>MGHHHHHHSHMNSCILQATVVEAPQLRYAQDNQTPVAEMVVQFPGLSSKDAPARLKVVGWGAVAQELQDRCRLNDEVVLEGRLRINSLLKPD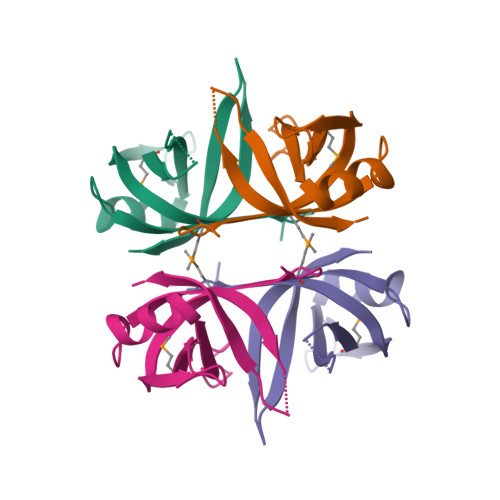GNREKQTELTVTRVHH[2x]>MSRVPEPSVFLVVDEAKRKARERGVGLIDLSIGSTDLPPPEAPLKALAEALNDPTTYGYCLKSCTLPFLEEAARWYEGRYGVGLDPRREALALIGSQEGLAHLLLALTEPEDLLLLPEVAYPSYFGAARVASLRTFLIPLREDGLADLKAVPEGVWREAKVLLLNYPNNPTGAVADWGYFEEALGLARKHGLWLIHDNPYVDQVYEGEAPSPLALPGAKERVVELFSLSKSYNLAGFRLGFALGSEEALARLERVKGVIDFNQYAGVLRMGVEALKTPKEVVRGYARVYRERALGMAEALKGVLSLLPPRATMYLWGRLPEGVDDLEFGLRLVERGV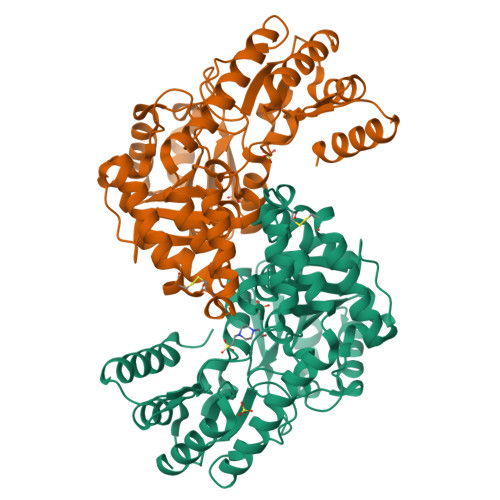ALAPGRGFGPGGKGFVRIALVRPLEELLEAAKRIREALD[2x]> MDEIDLRILKILQYNAKYSLDEIAREIRIPKATLSYRIKKLEKDGVIKGYYAYI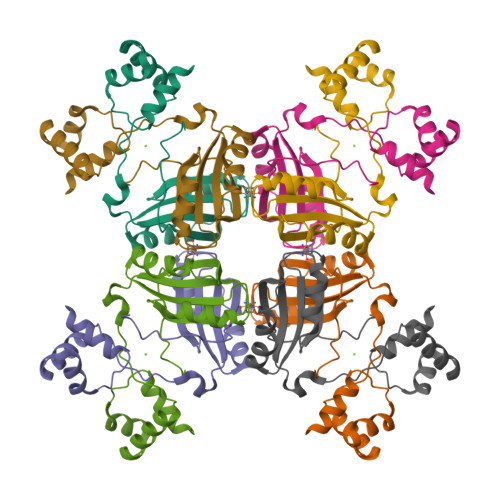NPASLNLDYIVITSVKAKYGKNYHVELGNKLAQIPGVWGVYFVLGDNDFIVMARYKTREEFMEKFLERVMSIPEVERTSTQVVVKIIKESPNIVIF>MATERTLSIIKPDAVAKNVIGEIESRFEKAGLKIVAAKMLQLSQEQAEGFYAEHKERPFFGDLVGFMTSGPVVVQVLEGENAIAANRDLMGATNPKEAEAGTIRADYAQSIDANAVHGSDSPESAAR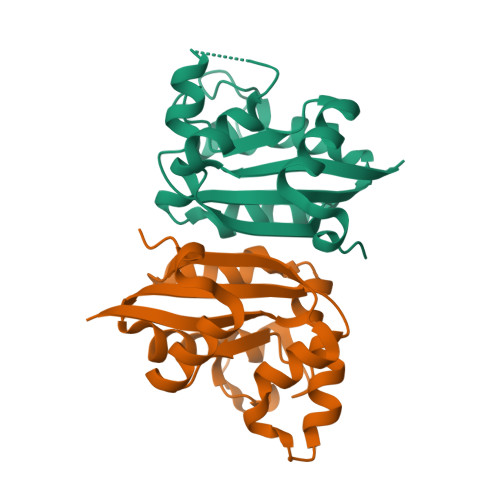EIAYFFAESEICSR[16x]> AYDRAITVFSPDGRLFQVEYAREAVKKGSTALGMKFANGVLLISDKKVRSRLIEQNSIEKIQLIDDYVAAVTSGLVADARVLVDFARISAQQEKVTYGSLVNI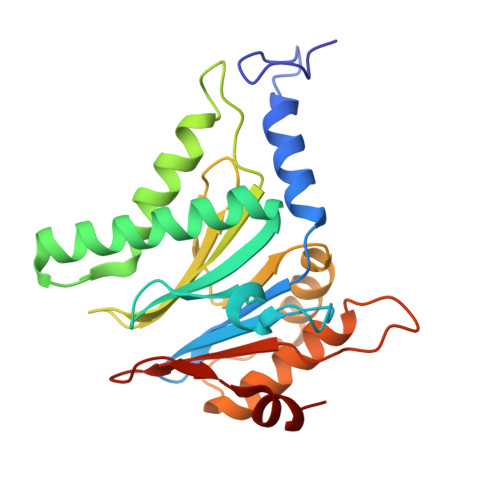ENLVKRVADQMQQYTQYGGVRPYGVSLIFAGIDQIGPRLFDCDPAGTINEYKATAIGSGKDAVVSFLEREYKENLPEKEAVTLGIKALKSSLEEGEELKAPEIASITVGNKYRIYDQEEVKKFL> ETGRTEAAPAAGQPVESFPLDFTAVEGNMDSFMAQVKSLAQSLYPCSAQQLNEDLRLHLLLNTSVTCNDGSPAGYYLKESRGSRRWLLFLEGGWYCFNRENCDSRYDTMRRLMSSRDWPRTRTGTGILSSQPEENPYWWNANMVFIPYCSSDVWSGASSKSEKNEYAFMGALIIQEVVRELLGRGLSGAKVLLLAGSSAGGTGVLLNVDRVAEQLEKLGYPAIQVRGLADSGWFLDNKQYRHTDCVDTITCAPTEAIRRGIRYWNGVVPERCRRQFQEGEEWNCFFGYKVYP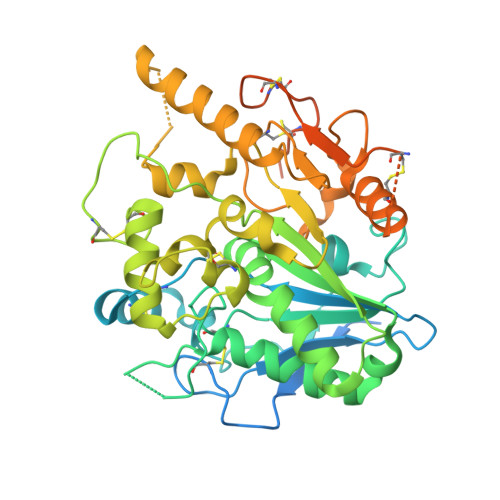TLRCPVFVVQWLFDEAQLTVDNVHLTGQPVQEGLRLYIQNLGRELRHTLKDVPASFAPACLSHEIIIRSHWTDVQVKGTSLPRALHCWDRSLHDSHKASKTPLKGCPVHLVDSCPWPHCNPSCPTVRDQFTGQEMNVAQFLMHMGFDMQTVAQPQGLEPSELLGMLSNGSGTKHHHHHH>[2x]RKPKTGILMLNMGGPETLGDVH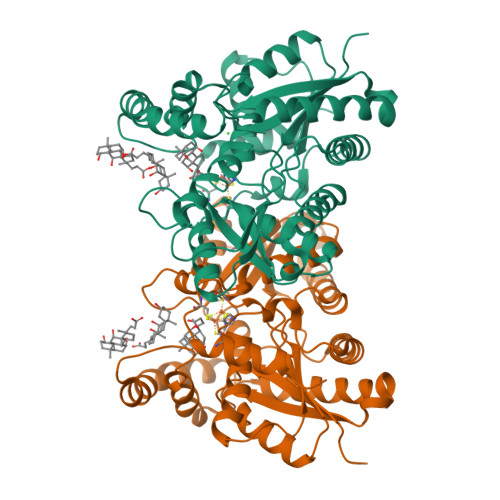DFLLRLFLDRDLMTLPIQNKLAPFIAKRLTPKIQEQYRRIGGGSPIKIWTSKQGEGMVKLLDELSPNTAPHKYYIGFRYVHPLTEEAIEEMERDGLERAIAFTQYPQYSCSTTGSSLNAIYRYYNQVGRKPTMKWSTIDRWPTHHLLIQCFADHILKELDHFPLEKRSEVVILFSAHSLPMSVVNRGDPYPQEVSATVQKVMERLEYCNPYRLVWQSKVGPMPWLGPQTDESIKGLCERGRKNILLVPIAFTSDHIETLYELDIEYSQVLAKECGVENIRRAESLNGNPLFSKALADLVHSHIQSNELCSKQLTLSCPLCVNPVCRETKSFFTSQQL>[4x]KIIMISGANSGIGHACIKYFLEKSFHVIALDINNNNLIDYMKTDMPLKVVQIDLSNSEAIHNLFTQLDLEKLSPDILINAAGIREITPVLHLSDDMFKKVIDVNLVAPFILSREVAKRWCESKIKGCIVNIASVSGLMAKPERAAYVASKHALIGLTKQMAMEFGKQNIRVNSISPGVIRTELTEEYFSNKALMSMIKSNQSLDTWGLPQDIVSCIEYLISDQARFITGSNFVI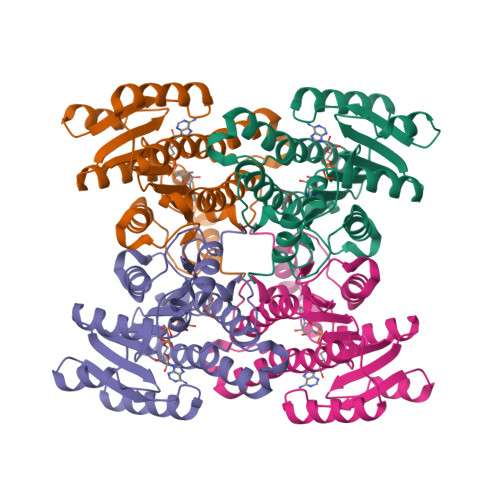DGGQTAGKNLLEKGELNSKLEGKPIPNPLLGLDSTRTGHHHHHH> SGEQKMAEAHELLKKFYHHLLINTKEGQEALDYLLSRGFTKELINEFQIGYALDSWDFITKFLVKRGFSEAQMEKAGLLIRREDGSGYFDRFRNRVMFPIHDHHGAVVAFSGRALGSQQPKYMNSPETPLFHKSKLLYNFYKARLHIRKQERAVLFEGFADVISAVSSDVKESIATMGTSLTDDHVKILRRNVEEIILCYDSDKAGYEATLKASELLQKKGCKVRVAMIPDGLDPDDYIKKFGGEKFKNDIIDASVTVMAFKMQYFRKGKNLSDEGDRLAYIKDVLKEISTLSGSLEQEVYVKQLASEFSLSQESLTEQLSVFS

Because DNA polymerases are incapable of initiating strand synthesis de novo, RNA primers are made by primase to prime DNA synthesis throughout replication; this priming activity is tightly coupled to the replisome by interactions with other replication partners. The DnaG primase is conserved in all bacteria and consists of three functional domains, an N-terminal zinc binding domain (ZBD), a central RNA polymerase domain (RPD) and a C-terminal helicase binding domain (HBD). Previous study indicated B. subtilis DnaG primase preferentially initiates primer synthesis at 5′-CTA-3′ sequence in template. To better understand the structure and function of primase and address the interactions between DnaG and specific DNA template, we have carried out structural and functional analysis on DnaG protein from B. subtilis (BsuDnaG).

Full length BsuDnaG was applied for crystallization trials and the structure of the RPD domain was solved. The results showed that proteolysis occurred in the crystallization drops and yielded a fragment of ~49 kDa. The crystals belonged to space group P61 with cell dimensions of a = b = 117.11 Å, c = 48.86 Å. There was one molecule per asymmetric unit. The RNA polymerase domain (RPD, residues 112–435) could be modeled in the electron density map. Superposition of RPD structure of B. subtilis against that of S. aureus, E. coli and A. aeolicus led to r.m.s.d. values of 1.31 Å, 1.80 Å and 1.73 Å, respectively. Clearly, the structure of BsuDnaG RPD shared similar overall structures with its homologs, except for a slight variation in the orientation of the C-terminal helical bundle. Structural comparison revealed that the orientation of loop1 in BsuDnaG RPD was quite different from that in ZBD/RPD of A. aeolicus; it appeared that the deletion of ZBD resulted in loop1 rotated about 25 degrees anti-clockwise. Our results show that the DnaG primase could degrade at the sites in the hinge regions.>[2x]SLFELGKMI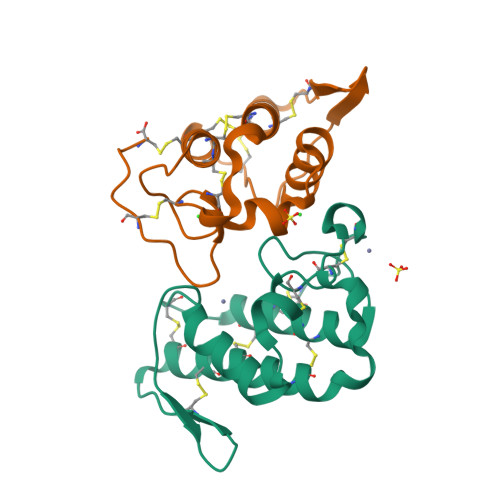LQETGKNPAKSYGAYGCNCGVLGRGKPKDATDRCCYVHKCCYKKLTGCDPKKDRYSYSWKDKTIVCGENNPCLKELCECDKAVAICLRENLGTYNKKYRYHLKPFCKLADPC5-methyl-3-phenyl-1,2-oxazole-4-carboxylic acid | C11 H9 N O3 | 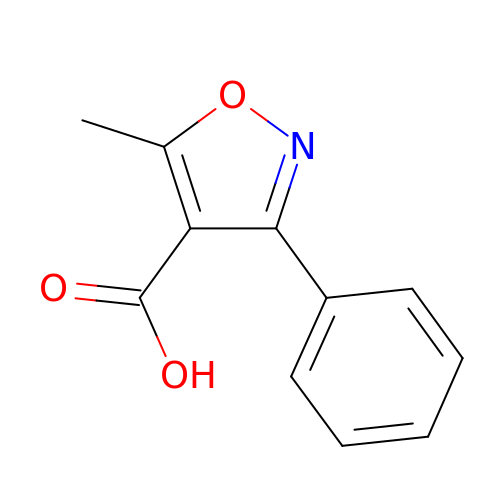PENHKTNQUJMHIR-UHFFFAOYSA-N>[6x]MSLRPQTSFIFDLDGTLTDSVYQNVAAWKEALDAENIPLAMWRIHRKIGMSGGLMLKSLSRETGMSITDEQAERLSEKHAQAYE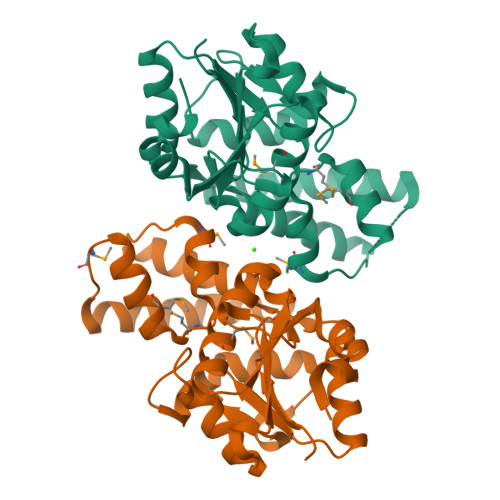RLQHQIIALPGAVELLETLDKENLKWCIATSGGIDTATINLKALKLDINKINIVTRDDVSYGKPDPDLFLAAAKKIGAPIDECLVIGDAIWDMLAARRCKATGVGLLSGGYDIGELERAGALRVYEDPLDLLNHLDEIASREGHHHHHH> 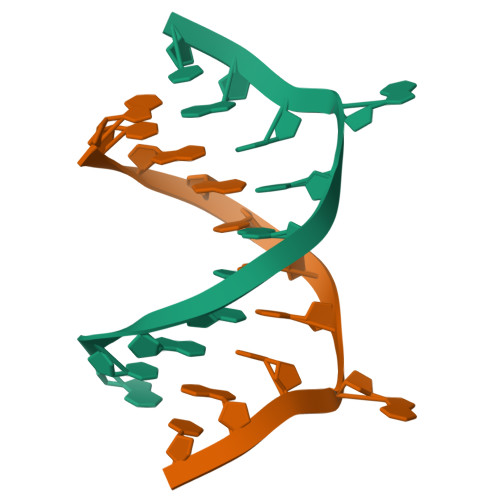GCGATATACGC>MAFSADTSEIVYTHDTGLDYITYSDYELDPANPLAGGAAWIEGAFVPPSEARISIFDQGYLHSDVTYTVFHVWNGNAFRLDDHIERLFSNAESMRIIPPLTQDEVKEIALELVAKTELREAFVSVSITRGYSSTPFERDITKHRPQVYMYAVPYQWIVPFDRIRDGVHAMV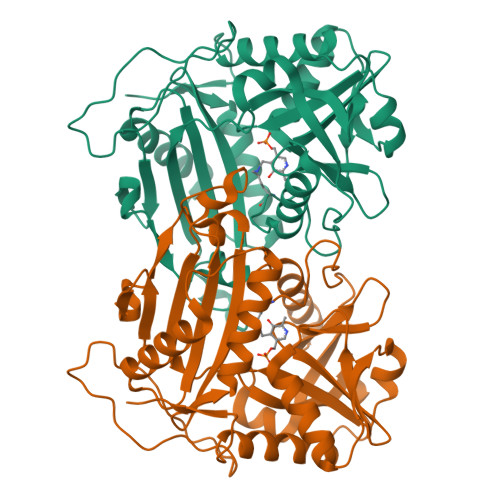AQSVRRTPRSSIDPQVKNFQWGDLIRAVQETHDRGFEAPLLLDGDGLLAEGSGFNVVVIKDGVVRSPGRAALPGITRKTVLEIAESLGHEAILADITLAELLDADEVLGCTTAGGVWPFVSVDGNPISDGVPGPITQSIIRRYWELNVESSSLLTPVQY[12x]>[4x]GSHMSAMAESKVLVKGTPFNKPVIKGKLENNYDMSQDEVSLLLFLKTHGGKIPLY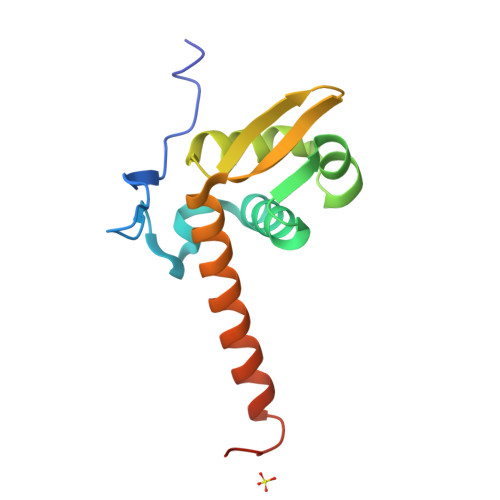RIKNETGLKDPESVLKNLMDYGFALEDKERLGEKIVLTSEGEFVAQAIRVRDEELRLKEMKQKKNVNRSSAPPQ> MQFSKMHGLGNDFMVVDAVTQNVFFSPELIRRLADRHLGVGFDQLLVVEPPYDPELDFHYRIFNADGSEVAQCGNGARCFARFVRLKGLTNKRDIRVSTANGR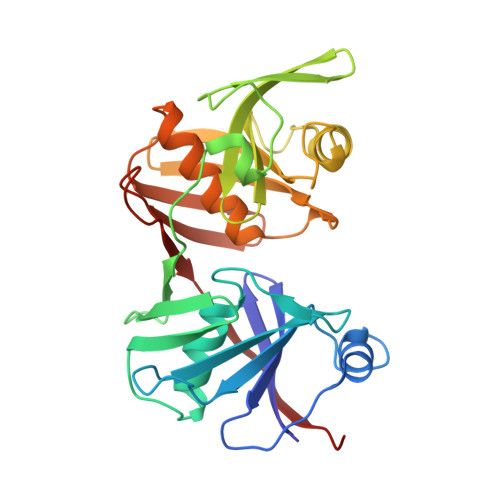MVLTVTDDDLVRVNMGEPNFEPSAVPFRANKAEKTYIMRAAEQTILCGVVSMGNPHCVIQVDDVDTAAVETLGPVLESHERFPERANIGFMQVVKREHIRLRVYERGAGETQACGSGACAAVAVGIQQGLLAEEVRVELPGGRLDIAWKGPGHPLYMTGPAVHVYDGFIHL> MRPARALIDLQALRHNYRLAREATGARALAVIKADAYGHGAVRCAEALAAEADGFAVACIEEGLELREAGIRQPILLLEGFFEASELELIVAHDFWCVVHCAWQLEAIERASLARPLNVWLKMDSGMHRVGFFPE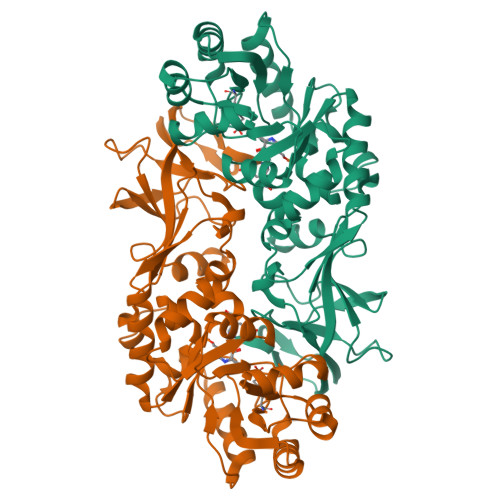DFRAAHERLRASGKVAKIVMMSHFSRADELDCPRTEEQLAAFSAASQGLEGEISLRNSPAVLGWPKVPSDWVRPGILLYGATPFERAHPLADRLRPVMTLESKVISVRDLPAGEPVGYGARYSTERRQRIGVVAMGYADGYPRHAADGTLVFIDGKPGRLVGRVSMDMLTVDLTDHPQAGLGSRVELWGPNVPVGALAAQFGSIPYQLLCNLKRVPRVYSGA> SGLCSDPAITYLKRLGYNVVRLPREGIQPLHLLGQQRGTVEYLGSLEKLITQPPSEPPAITRDQAAAGINGQKTENLSFSIGINILKSVLAQFGAGAGIEAQYNQARKVRFEFSNVLADSVEPLAVGQFLKMAEVDADNPVLKQYVLGNGRLYVITQVIKSNEFTVAAEKSGGGSIQLDVPEIQKVVGGKLKVEASVSSQSTVTYKGE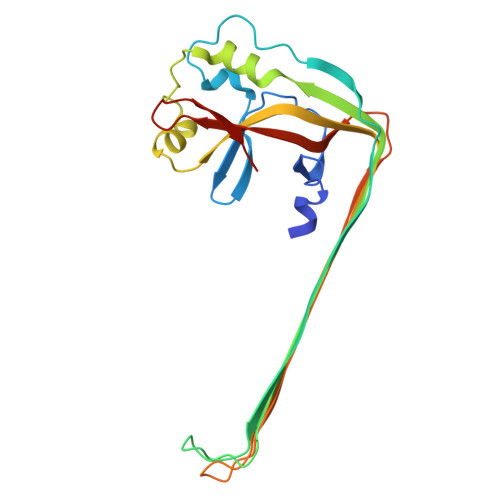KQLVFGFKCFEIGVKNGEITLFASQLVPR> GUGUGCCCGGCAUGGGUGCAGUCUAUAGGGUGAGAGUCCCGAACUGUGAAGGCAGAAGUAACAGUUAGCCUAACGCAAGGGUGUCCGUGGCGACAUGGAAUCUGAAGGAAGCGGACGGCAAACCUUCGGUCUGAGGAACACGAACUUCAUAUGAGGCUAGGUAUCAAUGGAUGAGUUUGCAUAACAAAACAAAGUCCUUUCUGCCAAAGUUGGUACAGAGUAAAUGAAGCAGAUUGAUGAAGGGAAA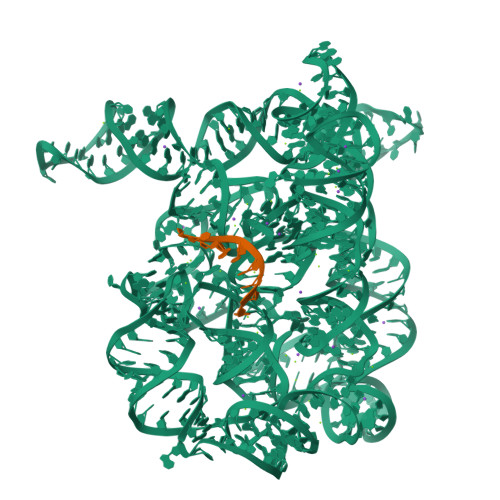GACUGCAUUCUUACCCGGGGAGGUCUGGAAACAGAAGUCAGCAGAAGUCAUAGUACCCUGUUCGCAGGGGAAGGACGGAACAAGUAUGGCGUUCGCGCCUAAGCUUGAACCGCCGUAUACCGAACGGUACGUACGGUGGUGUGAGAGGAGUUCGCUCUACUCUAU;> CGCUCUACUCUAU>HHHHHHSSGLVPRGSHMSARLSHVTVPVLDQDSAKEFYTEKLGFEVRNDMTMGGLRWLTVGPKDQPDVEMVLRRVGAPEYDEETAEQLRDLVAKGVIGVGVLHVDDTRATYERYRAAGVIFIQE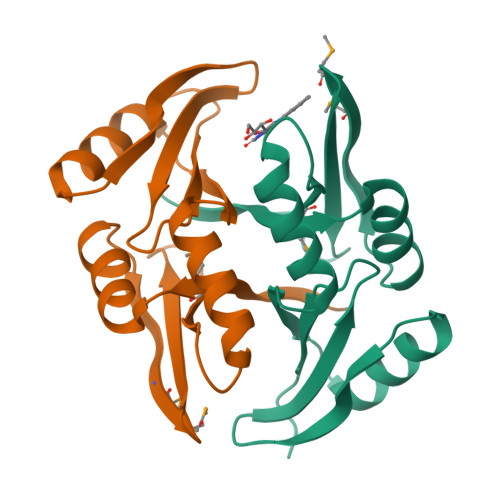PVKRPYGTEAVFRDDSGNWFSLTDARG[6x]>[14x]STSAGPTVPDRDNDGIPDSLEVEGYTVDVKNKRTFLSPWISNIHEKKGLTKYKSSPEKWSTASDPYSDFEKVTGRIDKNVSPEARHPLVAAYPIVHVDMENIILSKNEDQSTQNTDSQTRTISKNTSTSRTHTSEVHGNAEVHASFFDIGGSVSAGFSNSNSSTVAIDHSLSLAGERTWAETMGLNTADTARLNANIRYVNTGTAPIYNVLPTTSLVLGKNQTLATIKAKENQLSQILAPNNYYPSKNLAPIALNAQADFSSTPITMNYNQFLELEKTKQLRLDTDQVYGNIATYNFENGRVRVDTGSNWSEVLPQIQETTARIIFNGKDLNLVERRIAAVNPSDPLETTKPDMTLKEALKIAFGFNEPNGNLQYQGKDITEFDFNFDQQTSQNIKNQLAELNATNIYTVLDKIKLNAKMNILIRDKRFH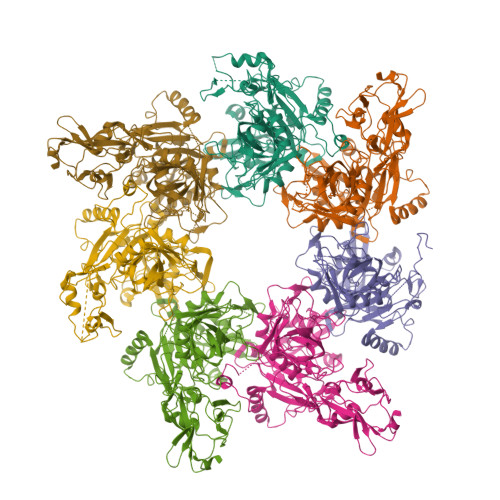YDRNNIAVGADESVVKEAHREVINSSTEGLLLNIDKDIRKILSGYIVEIEDTEGLKEVINDRYDMLNISSLRQDGKTFIDFKKYNDKLPLYISNPNYKVNVYAVTKENTIINPSENGDTSTNGIKKILIFSKKGYEIG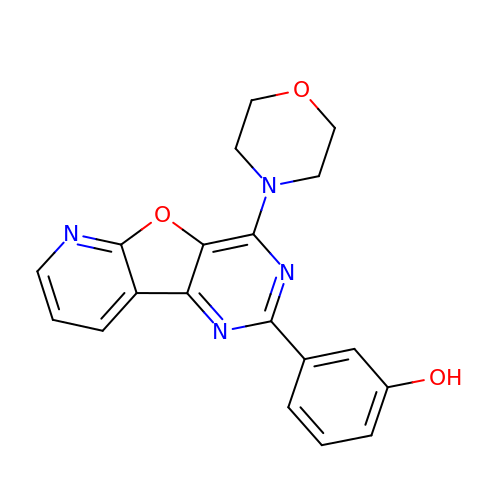3-(4-MORPHOLIN-4-YLPYRIDO[3',2':4,5]FURO[3,2-D]PYRIMIDIN-2-YL)PHENOL | C19 H16 N4 O3 | TUVCWJQQGGETHL-UHFFFAOYSA-N>[2x]MKFGLFFLNFMNSKRSSDQVIEEMLDTAHYVDQLKFDTLAVYENHFSNNGVVGAPLTVAGFLLGMTKNAKVASLNHVITTHHPVRVAEEACLLDQMSEGRFAFGFSDCEKSADMRFFN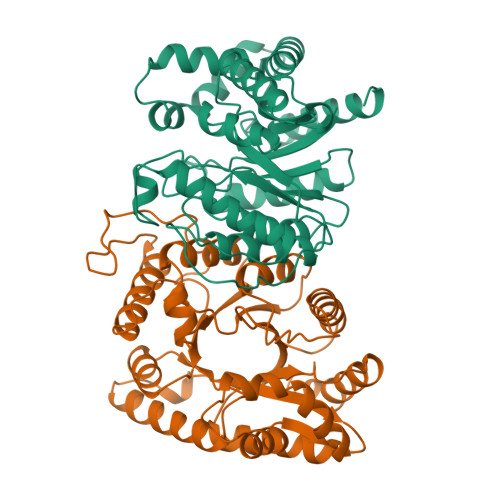RPTDSQFQLFSECHKIINDAFTTGYCHPNNDFYSFPKISVNPHAFTEGGPAQFVNATSKEVVEWAAKLGLPLVFRWDDSNAQRKEYAGLYHEVAQAHGVDVSQVRHKLTLLVNQNVDGEAARAEARVYLEEFVRESYSNTDFEQKMGELLSENAIGTYEESTQAARVAIECCGAADLLMSFESMEDKAQQRAVIDVVNANIVKYHS>[2x]TMSFFDLLNER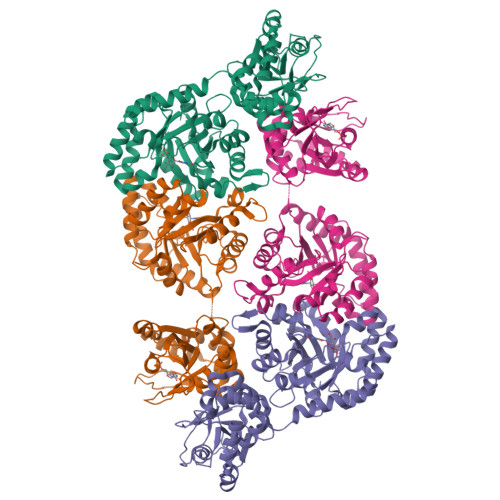AKRSLLCVGLDPRAKTAAAAVEECKRLIEQTHEYAAAYKPNAAFFEFFGAEGWAALSEVIRAVPAGIPVVLDAKRGDIADTADAYATSAFKHLNAHAITASPYMGSDSLQPFMRYPDKAVFVLCKTSNKGSNDLQCLRVGDRYLYEAVAERAEGPWNVNGNVGLVVGATDPVALARVRARAPTLWFLVPGIGAQGGSLKASLDAGLRADGSGMLINVSRGLARAADPRAAAKELCEEINAIRFAKGASVELAKALVDSHCVRFGNFTLKSGKSSPIYIDLRRLVTYPAIMRLVAREYAKVLRHYKFDRIAGLPYAALPIASAISNEMNVPLIYPRREAKIYGTKAAIEGEYKKGDRVVIIDDLVSTGETKVEAIEKLRSAGLEVVSIVVLVDRDMGAKAFLNKLGYDFEAVVGLHQLLPLWRKSNAITSQQEADVRAFLGQW AlkB homologue 5 (ALKBH5) is a ferrous iron and 2-oxoglutarate dependent oxygenase that demethylates RNA N6-methyladenosine (m6A), a post-transcriptional RNA modification with an emerging set of regulatory roles. We report three crystal structures of ALKBH5 in complex with an m6A-ssRNA 8-mer substrate and supporting biochemical analyses. Strikingly, the single-stranded RNA substrate binds to the active site of ALKBH5 in a 5′-3′ orientation that is opposite to single-stranded or double-stranded DNA substrates observed for other AlkB subfamily members, including single-stranded DNA bound to FTO. The results support a mechanism involving formation of an m6A hemiaminal intermediate, followed by efficient ALKBH5 catalyzed demethylation, enabled by a proton shuttle network involving Lys132 and Tyr139.

We modified the construct to produce N-terminally truncated ALKBH574–292 (residues 74–292); we were able to co-purify ALKBH574–292 in complex with Mn (substituting for Fe) and the m6A-containing 8-mer ssRNA substrate (U−3G−2G−1(m6A)0C+1U+2G+3C+4). Three copies of the ALKBH574–292–ssRNA complex are present in the asymmetric unit. Clear electron density is present for four (G−2G−1(m6A)0C+1) of the eight nucleotides of the ssRNA at the ALKBH5 active site region in all three copies in the asymmetric unit and the observable ssRNA does not appear to be involved in crystal contacts. Interestingly, in this initial substrate complex structure the ALKBH5 active site did not contain the cosubstrate 2OG analogue NOG, although NOG had been added to the sample mixture prior to purification by size exclusion chromatography. At the ALKBH5 active site in the structures reported here, a catalytically inert Mn ion (substituting for catalytically active Fe(II)) is coordinated by the highly conserved metal binding triad His204, Asp206, and His266, a water molecule, and either 2OG, NOG, or a sulfate ion. In the structure of the ALKBH574–292–RNA complex without 2OG or NOG, a sulfate ion (likely derived from the crystallization buffer) was observed to ligate to the Mn ion at the 2OG cosubstrate C-1 carboxylate binding site via one of its oxygens; the sulfate ion is also positioned to interact with Asn193 and Lys132. The observation of the Mn-ligating sulfate was unexpected because NOG was present in the initial complexation buffer.

>SQQLQKEEEARKVKSGIRQMRLFSQDECAKIEARIDEVVSRAEKGLYNEHTVDRAPLRNKYFFGEGYTYGAQLQKRGPGQERLYPPGDVDEIPEWVHQLVIQKLVEHRVIPEGFVNSAVINDYQPGGCIVSHVDPIHIFERPIVSVSFFSDSALCFGCKFQFKPIRVSEPVLSLPVRRGSVTVLSGYAADEITHCIRPQDIKERRAVIILRKTRLDAPRL[3x]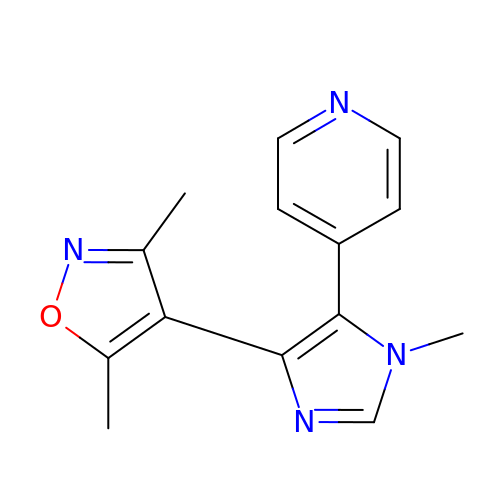3,5-dimethyl-4-(1-methyl-5-pyridin-4-yl-imidazol-4-yl)-1,2-oxazole | C14 H14 N4 O | XPQAEPLMWBAUIW-UHFFFAOYSA-N> GSHMASDLKNPYERIQAEAYDAMSGIQTEGTDDDGGGDNIGWINDGDWVKY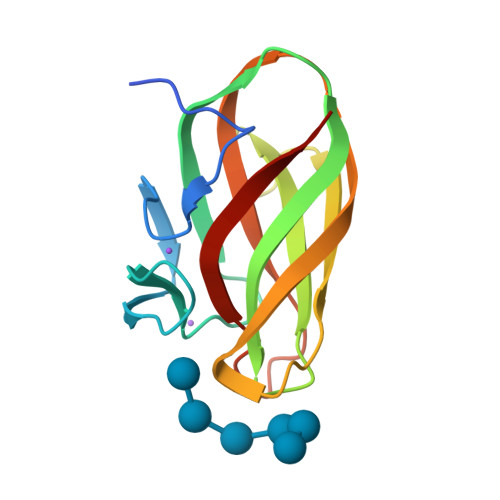ERVHFERDASSIEVRVASDTPGGRIEIRTGSPTGTLLGDVQVPNTGGWQQWQTVTGNVQIQPGTYDVYLVFKGSPEYDLMNVNWFVFRANG> MRGS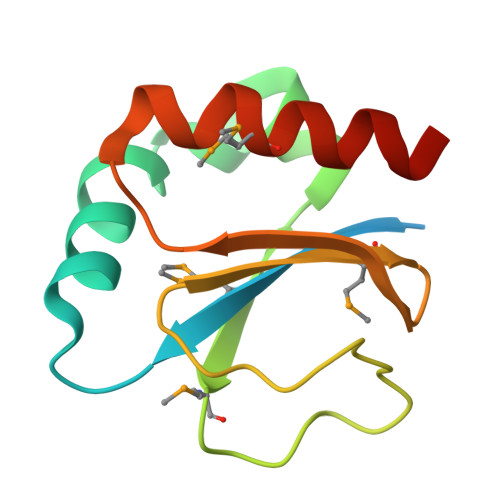HHHHHHGSDDDDKAELRLLMFEQPGCLYCARWDAEIAPQYPLTDEGRAAPVQRLQMRDPLPPGLELARPVTFTPTFVLMAGDVESGRLEGYPGEDFFWPMLARLIGQAEPGQ> SVTVPNDDWTLSSLSETFDDGTQTLQGELTLALDKLAKNPSNPQLLAEYQSKLSEYTLYRNAQSNTVKVIKDV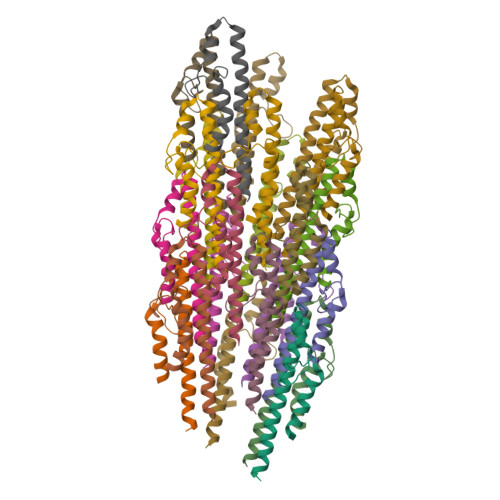DAAIIQNFR> SLQRVPSYDSFDSEDYPAALPNHKPKGTFKDYVRDRADLNKDKPVIPAAALAGYTGSGPIQLWQFLLELLTDKSCQSFISWTGDGWEFKLSDPDEVARRWGKRKNKPKMNYEKLS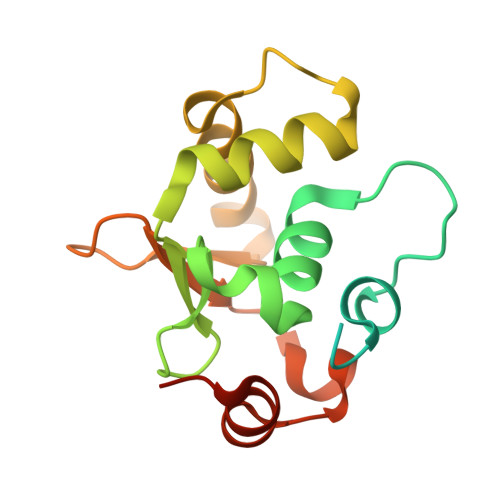RGLRYYYDKNIIHKTAGKRYVYRFVCDLQSLLGYTPEELHAMLDVKPDADE> GLGDELEEVIVEKTKQTVASISSGPKHTQKVPILTANETGATMPVLPSDSIETRTTYMHFNGSETDVECFLGRAACVHVTEIQNKDATGIDNHREAKLFNDWKINLSSLVQLRKKLELFTYVRFDSEYTILATASQPDSANYSSNLVVQAMYVPPGAPNPKEWDDYTWQSASNPSVFFKVGDTSRFSVPYVGLA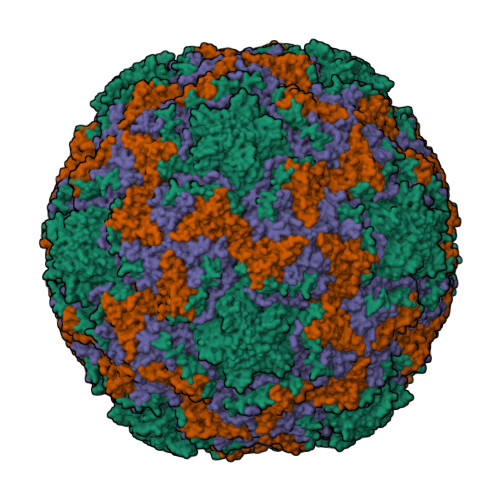SAYNCFYDGYSHDDAETQYGITVLAHMGSMAFRIVNEHDEHKTLVKIRVYHRAKHVEAWIPRAPRALPYTSIGRTNYPKNTEPVIKKRKGDIKSY;> SPNVEACGYSDRVQQITLGNSTITTQEAANAVVCYAEWPEYLPDVDASDVNKTSKPDTSVCRFYTLDSKTWTTGSKGWCWKLPDALKDMGVFGQNMFFHSLGRSGYTVHVQCNATKFHSGCLLVVVIPEHQLASHEGGNVSVKYTFTHPGERGIDLSSANEVGGPVKDVLYNMNGTLLGNLLIFPHQFINLRTNNTATIVIPYINSVPIDSMTRHNNVSLMVIPIAPLTVPTGATPSLPITVTIAPMCTEFSGIRSKSIVPQ;> GLPTTTLPGSGQFLTTDDRQSPSALPNYEPTPRIHIPGKVHNLLEIIQVDTLIPMNNTHTKDEVNSYLIPLNANRQNEQVFGTNLFIGDGVFKTTLLGEIVQYYTHWSGSLRFSLMYTGPALSSAKLILAYTPPGARGPQDRREAMLGTHVVWDIGLQSTIVMTIPWTSGVQFRYTDPDTYTSAGFLSCWYQTSLILPPETTGQVYLLSFISACPDFKLRLMKDTQTISQTVALTE;> GAQVSTQKSGSHENQNILTNGSNQTFTVINYYKDAASTSSAGQSLSMDPSKFTEPVKDLMLKGAPALN>MAQSSNSTHEPLEVLKEETVNRHRAIVSVMEELEAVDWYDQRVDASTDPELTAILAHNRDEAKEHAAMTLEWLRRNDAKWAEHLRTYLFTEGPITAANSSSVDKLAAALEHHHHHH[30x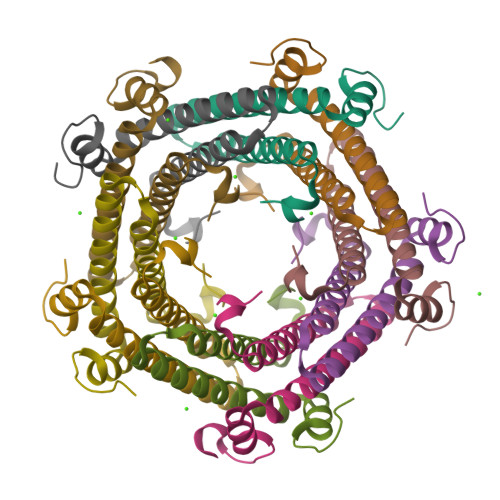]>[2x]SNAQREVRLPSGGSIVIDPTEALTSIDINSAR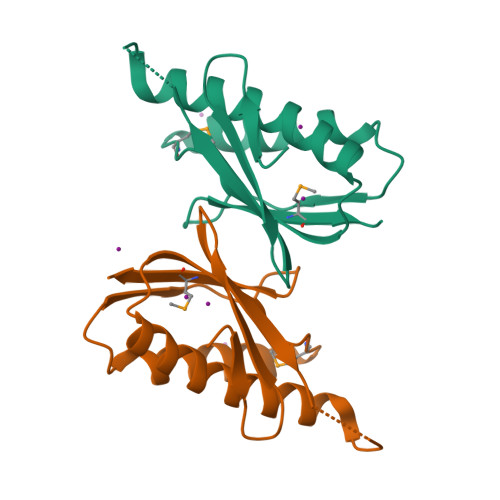ATKGGDIEETALNTNLEAADEIARQLRLRDLGGLVVIDFIDMTPVRHQREVENRLREAVRVDRARVQIGRISRFGLLEMSRQR Delta-3isotetradecenoic acid 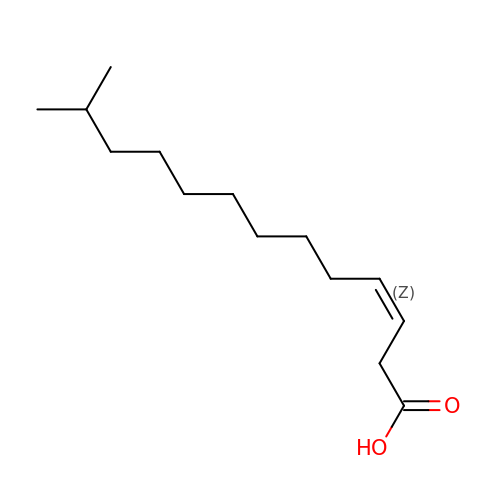| C14 H26 O2 | CPJZLQGGCFWOAA-NTMALXAHSA-N>[2x]ASNAPAPLAGVIFEPFQELKKDYLAVPIAHNVSLARQNYADDSESAINEQINVEYNVSYVYHALFAY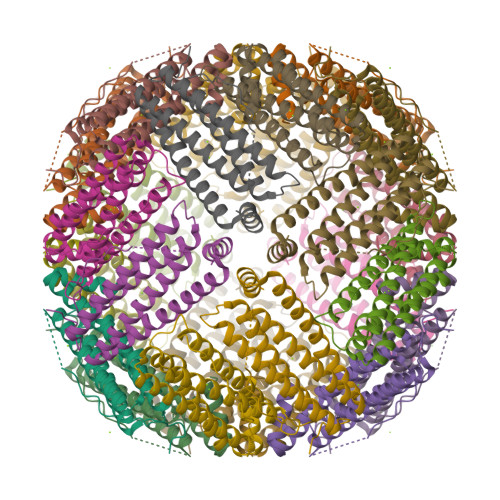FDRDNIALKGLAKFFKESSEEEREHAEQLIKYQNIRGGRVVLHPITSPPSEFEHSEKGDALYAMELALSLEKLTNEKLLHVHSVADRNNDPQLADFIESEFLYEQVKSIKKIAEYVAQLRLVGKGHGVWHFDQKLLHDEDHV>[4x]EEKEQKLQFVLRFGDFE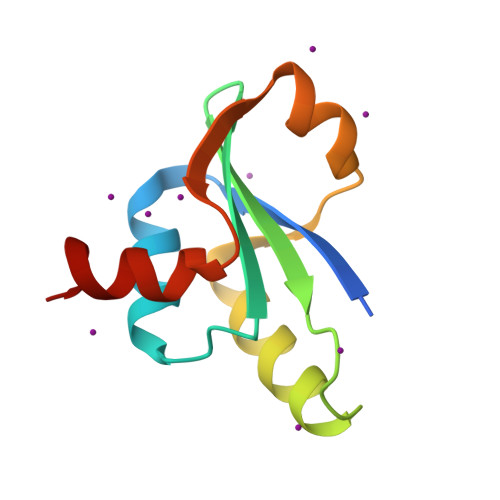DVISLSKLNVNGSKTTLYSFENRYYLYVDFCDMTDEEVENQLSIMLEYANESSISIHRLEEYGKLIISEHALETIKKHFAS> ANQLRELKQTHTYTVFGYTDGGFAVISADDLAPELLGVSESNFVETDNPSFKWWLKAIDEVITNAVKSNKPLNVI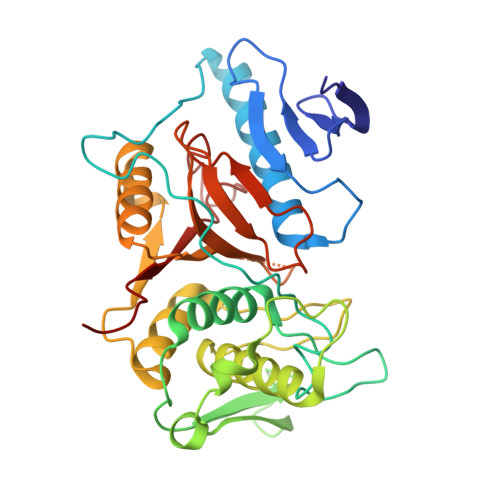KPDPSKYAAEVSTLLTTTWGQQMPYNKLLPKTKKGRLITGAVATATAQVLNYFKYPVRGIGSHTVHYPANDPSGVAISADFGNTTYDWANMKDNYSGNYTEAEANAVATLMLHCGVASEMQYGGPNEGSGAYMTDCAAGLRTYFGFTDAEYITRANYTDEQWMDIVFSELTKGHPLIYGGVSPGSMGQDAGHAFVIDGYNKAGLVSVNWGWNGDVDGYYKIDLLNPGNMYSFTAEQDMVRGVYGKP3-[2-fluoranyl-3-(trifluoromethyl)phenyl]-4-[[4-(methylamino)-6-propan-2-yl-quinazolin-2-yl]amino]benzoic 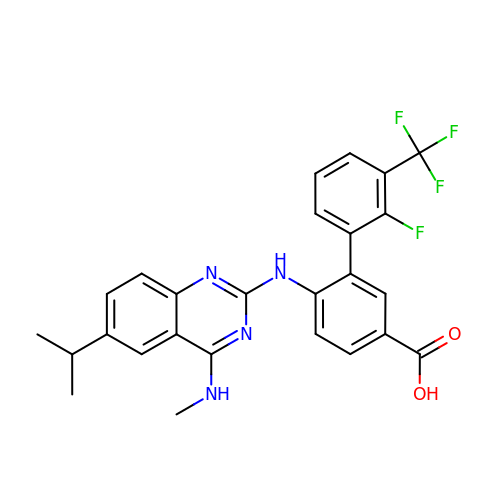acid | C26 H22 F4 N4 O2 | NVXLCRYRBAZDFU-UHFFFAOYSA-N>[2x]MARKYFVAANWKCNGTLESIKSLTNSFNNLDFDPSKLDVVVFPVSVHYDHTRKLLQSKFSTGIQNVSKFGNGSYTGEVSAEIAKDLNIEYVIIGHYERRKYFHETDEDVREKLQAS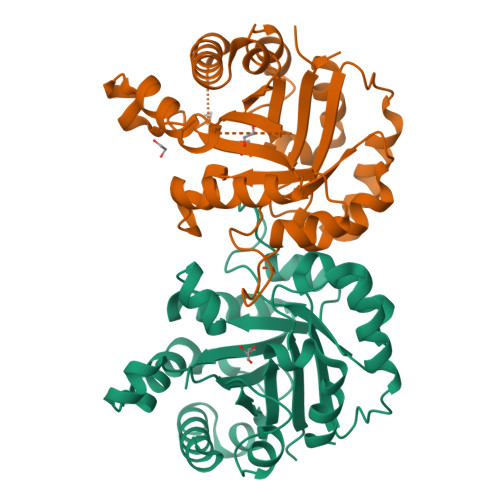LKNNLKAVVCFGESLEQREQNKTIEVITKQVKAFVDLIDNFDNVILVYEPLWAIGTGKTATPEQAQLVHKEIRKIVKDTCGEKQANQIRILYGGSVNTENCSSLIQQEDIDGFLVGNASLKESFVDIIKSAM> EQSSSEIKIVRDEYGMPHIYANDTWHLFYGYGYVVAQDRLFQMEMARRSTQGTVAEVLGKDFVKFDKDIRRNYWPDAIRAQIAALSPEDMSILQGYADGMNAWIDKVNTNPETLLPKQFNTFGFTPKRWEPFDVAMIFVGTMANRFSDSTSEIDNLALLTA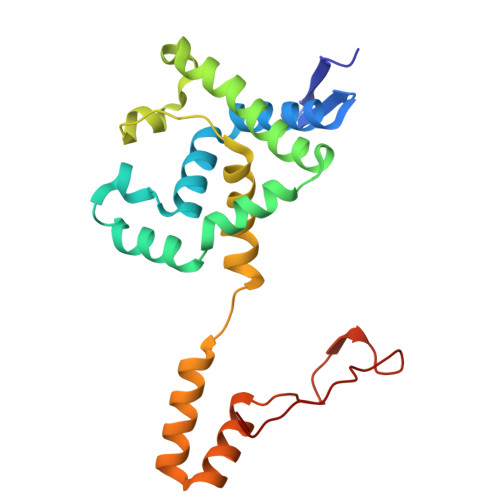LKDKYGVSQGMAVFNQLKWLVNPSAPTTIAVQESNYPLKFNQQNSQTA>QAKILEADAEILKAYAKILEAHAEILKAQ[106x]

Here we report seven high-resolution cryo-EM structures of filamentous peptide nanotubes based on a cross-α supramolecular architecture that provide insight into the designability of helical peptide filaments. A structural interaction is identified based on an appropriately placed pair of arginine residues (RxxxR) within the corresponding peptide sequences. This local interaction motif, designated as an arginine clasp, is robust within the context of these cross-α assemblies and can guide the coalescence of helical protofilaments into structurally defined cross-α nanotubes. In contrast to most structurally characterized filaments based on synthetic α-helical coiled-coils, the chain axes of the helical protomers are oriented in a plane nearly perpendicular to the long axis of the assembly.

In order to better compare the two models, cryo-EM data were collected on a fresh preparation of Form II filaments. Helical reconstruction afforded an atomic model at 4.2-Å resolution with a different helical symmetry (i.e., a rise of 1.93 Å and a rotation of 124.4°) than that proposed for the original model. The higher resolution model of Form II is consistent with a parallel orientation of the inner-outer helix pair, which was suggested but could not be unambiguously determined in the previous analysis. A structural comparison of the two assemblies indicated that helical protomers were arranged in four (Form I) or three (Form II) cross-helical stacks (i.e., protofilaments) that self-associated laterally to form single-walled and double-walled nanotubes, respectively. The main distinguishing feature between the Form I and Form II assemblies was the mode of lateral association between the respective cross α-helical stacks. Each nanotube was derived from coalesence of three protofilaments derived from the dimeric protomer. However, these were arranged in different symmetries; C3 for 29-20-2 and C1 for Form II. The main difference between the structures was manifested in terms of the lateral interactions between the termini of the protofilaments. These interactions occurred along the direction of the left-handed 12-start and 11-start helices for 29-20-2 and Form II, respectively, as illustrated in the the helical net diagrams of the corresponding assemblies. Among all three structures, the helices within the dimeric asymmetric unit could be superimposed with only minimal differences. Structural overlays of laterally interacting protofilaments indicated a conservation of the interfaces between the three filament structures.> MEYKSSPKRPYLLRAYYDWLVDNSFTPYLVVDATYLGVNVPVEYVKDGQIVLN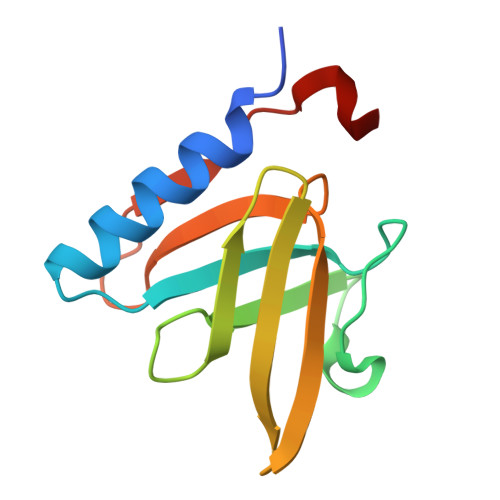LSASATGNLQLTNDFIQFNARFKGVSRELYIPMGAALAIYARENGDGVMFEPEEIYDE> MVSKAARRRRAAPRQQQRQQSNRASNQPRRRRARR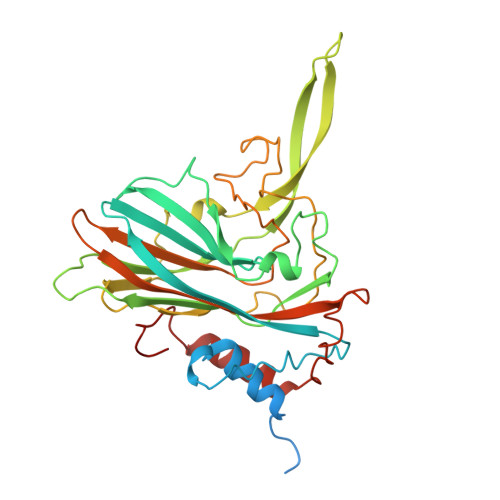TRRQQRMAATNNMLKMSAPGLDFLKCAFASPDFSTDPGKGIPDKFQGLVLPKKHCLTQSITFTPGKQTMLLVAPIPGIACLKAEANVGASFSGVPLASVEFPGFDQLFGTSATDTAANVTAFRYASMAAGVYPTSNLMQFAGSIQVYKIPLKQVLNSYSQTVATVPPTNLAQNTIAIDGLEALDALPNNNYSGSFIEGCYSQSVCNEPEFEFHPIMEGYASVPPANVTNAQASMFTNLTFSGARYTGLGDMDAIAILVTTPTGAVNTAVLKVWACVEYRPNPNSTLYEFARESPANDEYALAAYRKIARDIPIAVACKDN>[2x]MMNRIKKVLVANRGEIAIRVMRACTELKIKTVAIYSQEDTGSFHRYKSDEAYLVGAGKKPIDAYLDIENIIEIAKESGADAIHPGYGFLSENIEFAR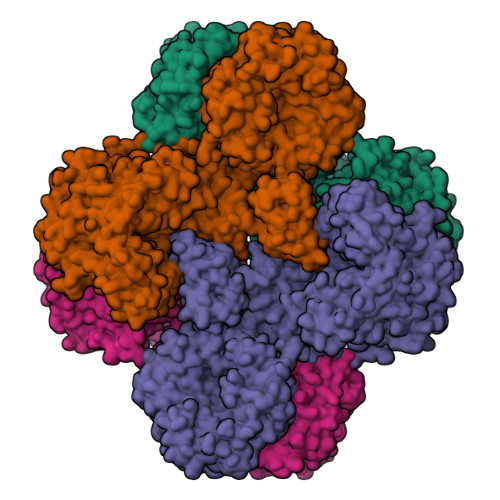RCEQEGIIFVGPKSKHLDMFGDKIKAKEQALLADIPVIPGSNGPVAGIKEVEEFGEKNGYPLMIKASLGGGGRGMRVVESKEHVKESFERASSEAKAAFGNDEVYVEKCVMNPKHIEVQILGDTHGNIVHLFERDCSIQRRHQKVVEVAPCNAITSELRNRICDAAVKLMKNVDYINAGTVEFLVEGDDFYFIEVNPRVQVEHTITEMITGIDIVQSQLFIADGYALHDQLVAIPKQEDIHIHGSAIQSRITTEDPLNNFMPDTGRVDTYRSTGGFGVRLDAGNGFQGTVVTPFYDSLLVKLCTWGMTFEQATRKMRRNLIEFRIRGVKTNIPFLLNVVRHPDFASGNYNTSFIDTTPELFKFPHIRDRGTKTLRYIGNVTVNGFPGIKHRDKPVYAEPRLPKIPYGSQISPGTKQILDAKGPEGVVDWVKKQEEVLLTDTTLRDAHQSLLATRVRSKDIFQIADAMAHLLPNMFSFEMWGGATFDVAYRFLNEDPWVRLETLRKQIPNVMFQMLLRGANAVGYKNYPDNVIREFVKQSAQSGVDVFRVFDSLNWIKGMEVSIDAVREAGKIVEAAICYTGDIDDDTRTKYTIDYYKDMAKELVAQGTHILGIKDMAGLLKPQAAYRLIGELKDTVDVPIHLHTHDTSGNGIYTYAAAVSAGVDIVDVASSAMSGATSQPSMTGLYYGLVNGNRQTNLDAQNSQIINHYWEDVRHYYKDFDNALNSPQTEVYIHEMPGGQYTNLQQQAIAVGLGDRWDEVKEMYTVVNQMFGDIVKVTPSSKVVGDLALFMVQNELSEEDVYEKGDTIDFPDSVIEFFMGEIGQPYGGFPEKLQKLVLKGRTPLTDRPGALMEPVNFVEVKAELKEKMGYEPTEKDVISYILYPKVFLDYQEMINKYGDVTVLDTPTFYKGMRLGETIEVELEKGKILLIKLNSIGEPIADGTRVIYFELNGQPREINIQDMNVQSTVIARRKIDTTNPEHVGATMTGSVIQVVVKKGDSVKKGDPLLITEAMKMETTIQAPFDGEVSSIYVSDGDTIESGDLLIEVNRI>[2x]SNAMTAPRAWRPIAGGPPAGPLVLAVDFAATGRPEAAFADLVARLDPGTEVWESLQPPLGTETGMVAEDYVTRWEEEVRASGRRIGAVLGFCAGSAFAGELAVRLARSQPRSPRLVV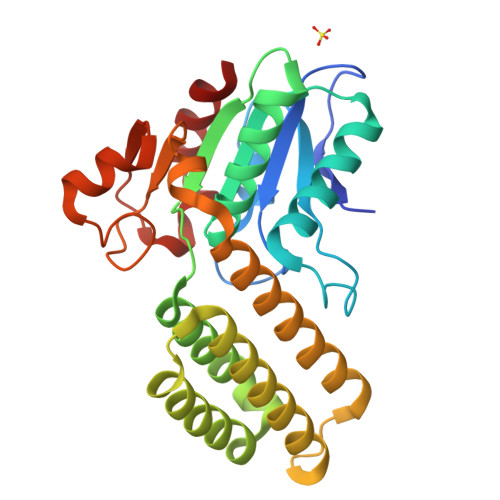FDPESPTTSTLYYQFRKVVESLAGVLGEQAAREALAEGTAAADRIGDVEGLGAELVRVFTAAGRAACAAADLDDEFADELTATYRSFVSYLVAAAAVDHVKCWSGAVAVSSATPTSGLNPLDPAARAALVERELTFDVHHADLLRDPGVARAVARLLA>[4x]HMAEIYLAGGCFWGLEEYFSRISGVLETSVGYANGQVETTNYQLLKETDHAETVQVIYDEKEVSLREILLYYFRVIDPLSINQQGNDRGRQYRTGIYYQDEADLPAIYTVVQEQERMLGRKIAVEVEQLRHYILAEDYHQDYLRKNPSGYCHI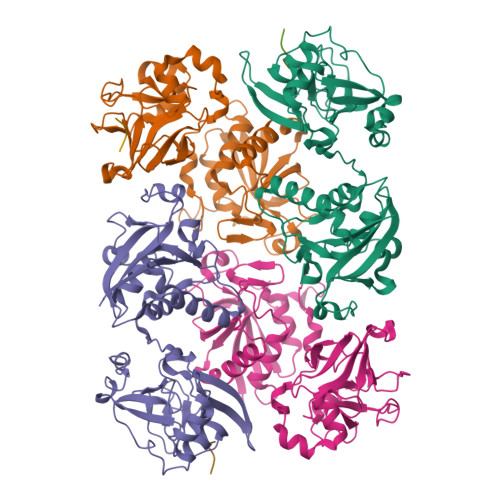DVTDADKPLIDAANYEKPSQEVLKASLSEESYRVTQEAATEAPFTNAYDQTFEEGIYVDITTGEPLFFAKDKFASGCGWPSFSRPLSKELIHYYKDLSHGMERIEVRSRSGSAHLGHVFTDGPRELGGLRYCINSASLRFVAKDEMEKAGYGYLLPYLNK;>SHMAEI[3x]>GSHM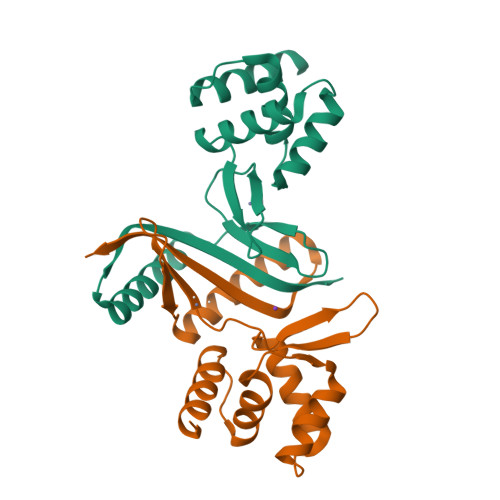ASMKDSYERSKKILEDAGINVTVQRLQMANLLLSKPQHLTADQVFQLINEHMPNASRATIFNNLKLFAEKGIVNLLELKSGITLYDSNVIHHHHAIDEKTGEIYDISLDSKLQEKVLSELKQDFKLKTGSSLENCNLSITLKGKKNP[2x]>NNQDERRALLERCLKGEGEIEKLQTKVLELQRKLDNTTAAVQELGRENQSLQIKHTQALNRKWAEDNEVQNCMACGKGFSVTVRRHHCR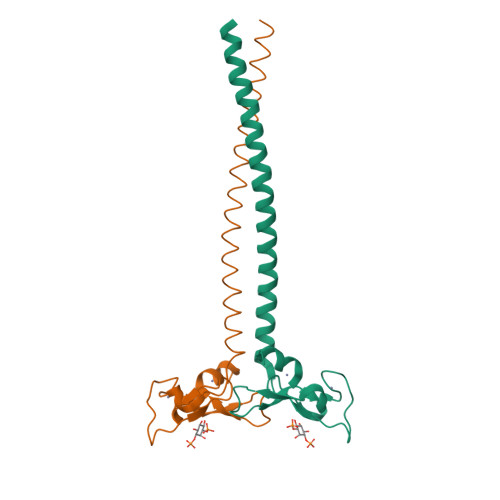QCGNIFCAECSAKNALTPSSKKPVRVCDACFNDLQG[2x]> GSHMGSQFWVTSQKTEASERCGLQGSYILRVEAEKLTLLTLGAQSQILEPLLFWPYTLLRRYGRDKVMFSFEAGRRCPSGPGTFTFQTSQGNDIFQAVEAAIQQQKAQGKVGQAQDILRLEHHHH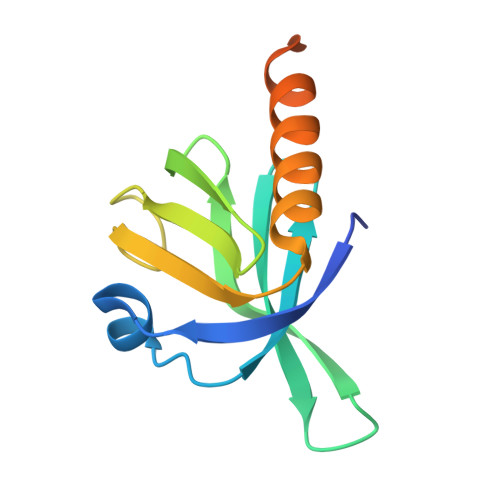HH>[2x]MLRSTHSPSGSSSAAPASSS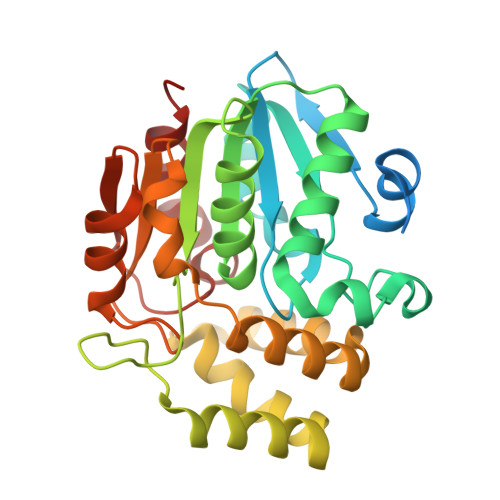SDAAMVGGGGAAAAAGSGGAPSGAKLLQILNVRVVGNGDRVVVLSHGFGTDQSAWSRVLPYLTRDHRVVLYDLVCAGSVNPEHFDFRRYDTLDSYVDDLLAILDALRIPRCAFVGHSVSAMIGILASIRRPELFAKLVLIGASPRFLNDNDYHGGFELPEIQQVFDAMAANYSAWAVGYAPLAVGADVPAAVQEFSRTLFNMRPDISLHVCRTVFNTDLRGVLGMVRSPCVVVQTTRDVSVPASVAAYLRAHLGGRTTVEFLQTEGHLPHLSAPGLLAQVLRRALARY>[4x]MQIYHTDVLCIGGALAGERVAVEASMAGLKTIMLSLVPPRRSHSSAAQGGMQAALGNAIMGDGDSPDVHFADTVKGSDWGCDQEVARIFADTAPIVMREVAHWGVPWNRVVPGKHTYYKGGKPFEAEEKAEKAGLIHARAFGGTAAWRTCYTADGTGRSVLNTLDTKCLQYGVTVHDRMQAEALIHDGGNCLGCIARCLRTGELVAYLATSTLIATGGYGRIYKATTNAVICDGGGQIIALDTGLVPMGNMEAVQFHPTGTVPTDILVTEGCRGDGGTLLDVNQYRFMPDYEPDKAQLASRDVVSRRMTEHMRKGLGVKSPYGDHLWLDIRHLGEKHITTKLREVYDICTNFLGVNPIHQLIPVRPTHHYSMGGVRTNRDGAAYGLKGLFSAGESACWDMHGFNRLGGNSLAETVVAGRYIGERMVEFTKGATPSFGMQYVEDAHKKVQERITDIVTGRKGKENTFKIRDEMHDIMMEGVGIFRNGTDLQKAVNKLEELYDRSQKISLSSACKGMNPELSTALRIRGMLKLAQCTAYGALDRTESRGAHTREDFPERNDKEWLNRTLSYWKEGASMPTLEYEEASPYYEMPPGDRGYGGGVTIANELPPEKFVIPEAAKENLKKAKL;>[4x]MNRMLTLNIFRYNPLDPDSQPRMQTFTVQEYDSMTLFIALTQIRDEKDPTLKVDFCCRAGICGSCAMVINGRPGLACHTQTKDLPAEITLHPLPFFQLLGDLSVDTGSWFRKTGLQIEAWCHSDDKAFDPTADEMRMDNDLANEIFELDRCIECGCCVAACGTARMRTDFLGAVSIMRVARFYLDPRDKRSEDDYYDVIGNDQGVFGCMGLLACEDVCPKGIPLQDQLGIMRRMMAMHSVKGVLPRPLIETIKKKGCCHAHAQS;>MNASTITLHVPQRSKIAGRMDFFQMVSGALLILFLWAHMMLVSSVILSPSLMNGIAWFFEATYMAQIGGPAVFVLMVVHFILAARKMPFKQDEWKTFRVHACMLHHKDTTMWVVQVISAIFILVLGAVHMFVVLTDLPITAAKSAARLQSGWLYLYLVLLPLAELHVGVGFYRIGVKYGFVGRNKRKWFQKTENLMMIGFITIGLLTLVRFMLLNIQG[4x]

One of these crucial enzymes is quinol:fumarate reductase (QFR), which is an integral membrane protein with three subunits: a flavoprotein (subunit A), an iron-sulphur protein (subunit B), and a membrane-embedded subunit (subunit C). QFR catalyzes the coupled reduction of fumarate to succinate with the oxidation of hydroquinone (quinol) to quinone on opposite sides of the inner cytoplasmic membrane. We have determined the crystal structure of QFR from D. gigas at 3.6 Å resolution by X-ray crystallography. All the redox cofactors and a bound menaquinone are revealed in our structure.

Two hetero-trimeric complexes, each comprising subunits A, B and C, form one stable homo-dimer (A2B2C2) with major contacts between two C subunits. The main driving force in the homo-dimer formation thus comes from interactions between the C subunits. The C8M methyl group of the flavin of FAD binds to the FAD-binding domain through a covalent bond with residue His-A43, which is conserved among these A subunits of QFRs. A fumarate molecule is also observed near the FAD in the A subunit. The high-potential heme bH is proximal to the hydrophilic A and B subunits, and has as axial ligands His-C79 and His-C166 on helices α3 and α6, respectively. The low-potential heme bL, which is located distal to the hydrophilic A and B subunits, is coordinated to His-C38 and His-C129 on helices α1 and α5, respectively. One n-dodecyl β-D-maltoside (DDM) molecule from the detergent used to solubilize and stabilize the protein is found in subunit C of D. gigas QFR. Instead, we have identified a new bound menaquinone near helix 1 and heme bL in the QFR structure of D. gigas. The Tyr-C63 that binds MK exhibits the lowest B-factor compared to the three other free Tyr63 residues of the asymmetric subunits C (i.e., G-chain, K-chain and O-chain), which might result from the formation of the hydrogen bond between the side-chain O–H of the C-chain Tyr-C63 and the bound MK. We propose that this bound menaquinone (MK) serves as a novel redox cofactor, or a coupling site to gate the proton-coupled electron transport across the membrane in D. gigas QFR.> SDYVHEVPPPGEIVRPPIQLGETYYAVKNKAIASWVSIKVIEFTESTAINGNTMKSYKIRYLNTPYQMIKTVTAKHIAYFEPPPVRLTIGTRVIAYFDGTTLSRGKDKGVVQSAFYPGIIAEPLKQANRYRYLIFYDDGYTQYVPHRDVRLVCQASEKVWEDVHAASRDFIQKYVEKYSVDRPMVQCTRGQSM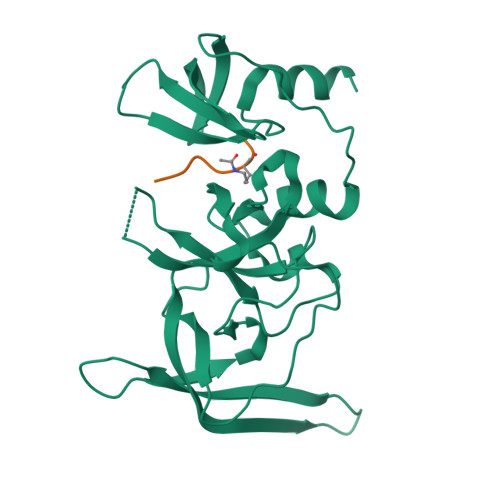TTESNGTWLYARVIDIDCSLVLMQFEGDKNHTEWIYRGSLRLGPVFRETQNNMNSSSAQQLRVP;> TKQTARKSTGGKAPRKQ>GPGSGGSGERKISRIHLVSEPSITHFLQVSWEKTLESGFVITLTDGHSAWTGTVSESEISQEADDMAMEKGKYVGELRKALLSGAGPADVYTFNFSKESCYFFFEKNLKDVSFRLGSFNLEKVENPAEVIRELICYC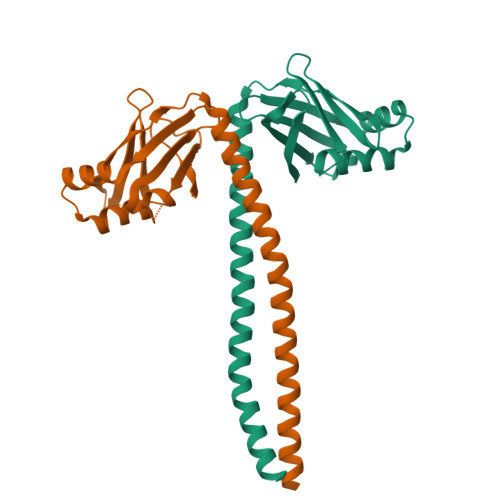LDEIKSLKHEIKELRKEKNDTLNNYDTLEEETDDLKNRLQALEKEL[2x]>[2x]MKIEPITGSEAEAFHRMGSRAFERYNEFVDLLVGAGIADGQTVVDLCCGSGELEIILTSRFPSLNLVGVDLSEDMVRIARDYAAEQGKELEFRHGDAQSPA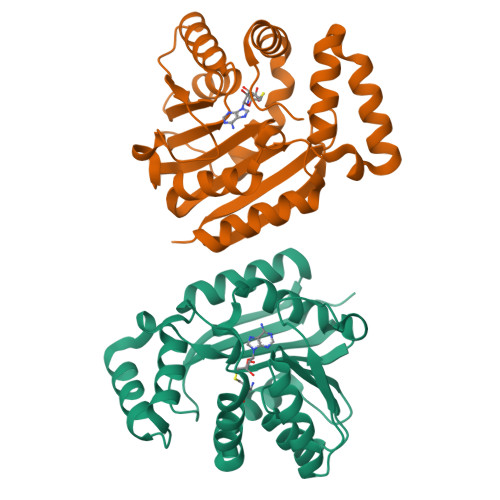GMEDLLGKADLVVSRHAFHRLTRLPAGFDTMLRLVKPGGAILNVSFLHLSDFDEPGFRTWVRFLKERPWDAEMQVAWALAHYYAPRLQDYRDALAQAADETPVSEQRIWVDDQGYGVATVKCFARRAAA> MGSSHHHHHHSSGLVPRGSHPSLRTQPSLYSGPFPF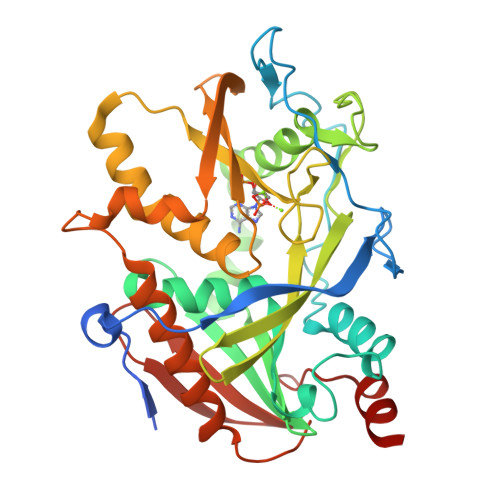YRRPSELGCFSLDAQRQYHGDARALRYYSPPPINGPGPDFDLRDGYPDRYQPRDEEVQERLDHLLRWVLEHRNQLEGGPGWLAGATVTWRGHLTKLLTTPYERQEGWQLAASRFQGTLYLSEVETPAARAQRLARPPLLRELMYMGYKFEQYMCADKPGGSPDPSGEVNTNVAYCSVLRSRLGNHPLLFSGAVDCLNPQAPCTQPPSCYVELKTSKEMHSPGQWRSFYRHKLLKWWAQSFLPGVPHVVAGFRNPEGFVCSLKTFPTMEMFENVRNDREGWNPSVCMNFCAAFLSFAQSTVVQDDPRLVHLFSWEPGGPVTVSVHRDAPYAFLPSWYVETMTQ>[2x]SAPAQEHPEATVLFSDIVGFTEIASRSSPLEVCSLLDELYQRFDAAIEEYPQLYKVETIGDAYMVVCNVTVPCDDHADVLLEFALRMHEEASRVASSLGEPVRIRVGMHSGPVVAGVVGRKMPRFCLFGDTVNTASRMESHGEAGQIHISEACYCCLRSKERFEIRERGNITVKGKGTMRTYLLSPLERT

Here, we report the structure of the catalytic domain of a soluble guanylate cyclase (CYG12) from the unicellular green algae Chlamydomonas reinhardtii, which shares 40 to 50% identity with the soluble and membrane-bound guanylate cyclase catalytic domains. The 991-residue full-length CYG12 protein contains each of the domains present in well-characterized soluble guanylate cyclases as well as an additional C-terminal domain of unknown function, and has the full complement of residues necessary to function as a homodimer. Each guanylate cyclase domain contains a central seven-stranded β sheet surrounded by several α helices. The two monomers in the wreath-like dimer are related by a twofold axis, and a central cleft, formed by the dimer interface, contains the two symmetric active sites.

The three C-terminal residues of each monomer are disordered, as are residues 564–566 in monomer A and residues 562–565 in monomer B. The final model of the guanylate cyclase dimer includes residues 467–563 and 567–653 for monomer A and residues 467–561 and 566–653 for monomer B. The model also includes 8 phosphate ions and 99 solvent molecules, and was refined to 2.55 Å resolution. During refinement, we observed unexplained peaks in electron density maps around five of the fourteen cysteine residues in the dimer (Cys 499 and Cys 592 of both monomers, and Cys 621 of monomer B). We wondered whether the apparent modification of the cysteine sidechains might be due to the addition of dimethylarsenic groups via reaction of the cysteine thiol group with the sodium cacodylate [sodium dimethylarsenate, (CH3)2AsO2Na] buffer and dithiothreitol reductant present during crystallization. We will focus on one active site, and refer to each domain as monomer A or B. In the C. reinhardtii guanylate cyclase described here, the catalytic residues are the metal-binding residues Asp 482(A) and Asp 527(A) located in the β2–β3 loop and in strand β1b, respectively, the ribose-orienting residue Asn 599(B) and the transition-state-stabilizing residue Arg 603(B), both located in helixα4, and the triphosphate-positioning residues Arg 571(A) in strandβ4a and Lys 640(B) in the β7–β8 loop. In our structure, the corresponding residues are Glu 523(B) and Cys 592(B), which are situated close to the locations of their adenylate cyclase counterparts. For Cys 592(B), the dimethylarsenic modification of the thiol side chain prevents potential hydrogen bonding interaction with the exocyclic carbonyl group of a substrate GTP molecule. The modification also results in distortion of the β2–β3 loop that contains the metal-binding residue Asp 527(A) and the base-recognition residue Glu 523(A), causing it to adopt a conformation incompatible with binding a metal-nucleotide complex. Comparison of our guanylate cyclase catalytic domain structure to structures of the mammalian adenylate cyclase suggests that the guanylate cyclase catalytic domain is in an inactive conformation.>VTQVGF[2x]

Curli proteins are produced via dedicated and tightly regulated cellular processes, and their fibrils mediate host cell adhesion and invasion, lead to immune system activation, and scaffold bacterial communities known as biofilms. The two key players in curli fibril formation are CsgA and CsgB, the major and minor curli subunits, respectively. CsgA, a 151-residue protein, consists of five imperfect sequence repeats (R1-R5), defined by regularly spaced serine (Ser), glutamine (Gln) and asparagine (Asn) residues. The first and the last repeats (R1 and R5) form amyloid fibrils in isolation and are critical to CsgA seeding and nucleation by CsgB, while the other repeats (R2-R4) contain 'gatekeeper' residues that temper the amyloidogenicity of CsgA.

However, while 45LNIYQY50 (R1), 47IYQYGG52 (R1), and 137VTQVGF142 (R5) formed unbranched and elongated amyloid-like fibrils, the 129TASNSS134 (R4-R5 loop) segment formed scarce and more amorphous structures. The 45LNIYQY50 (R1), 47IYQYGG52 (R1), and 137VTQVGF142 (R5) segments bound the amyloid indicator dye ThT and demonstrated dose-dependent amyloid fibrillation curves with short lag times. 45LNIYQY50 and 47IYQYGG52, which are overlapping segments from the R1 repeat, adopted very similar structures. Both segments, as well as 137VTQVGF142 (R5), adopted a classical amyloid steric zipper architecture, with two possible dry interfaces between paired β-sheets. The β-strands were oriented parallel to each other along the β-sheets. These three structures are class 1 steric zippers, as defined by Sawaya and Eisenberg according to the organization of the β-strands and β-sheets. In each of these dry interfaces, the chemical properties governing fibril stability, i.e., buried surface area and shape complementarity between sheets, resembled those of eukaryotic steric zipper structures. Specifically, the R1 45LNIYQY50 and 47IYQYGG52 segments and the R5 137VTQVGF142 segment formed fibrils that bound the amyloid indicator dye ThT and formed canonical amyloid class 1 steric zippers. These segments contain Gln49 or Gln139 (marked in bold in 45LNIYQY50, 47IYQYGG52, and 137VTQVGF142), which are critical for fibrillation and cannot be mutated to asparagine without interfering with curli assembly. The R1 segment 45LNIYQY50 and the R5 segment 137VTQVGF142 also induced fibrillation of Aβ1–40. In agreement with the hypothesis that the steric zipper segments serve as spines of CsgA fibrils, we found that the D-peptides also inhibited the fibrillation of the R1 45LNIYQY50 and R5 137VTQVGF142 spine segments in a dose-dependent manner.> MTKYELKMQYFDEWMIRWRKFQTESDWEIEKGRQWWRRFNMAVSGALFCGLVLYTSGTATLKRQYGLPHF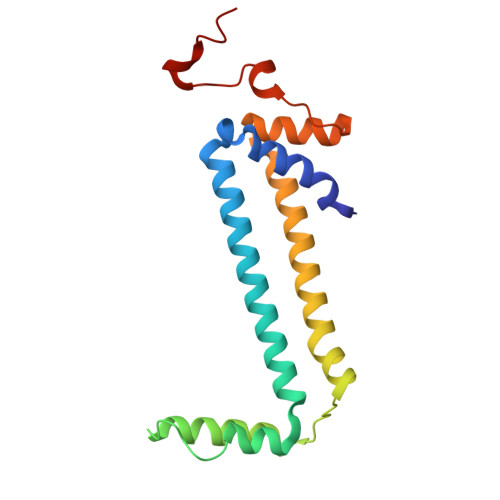FDIGVDGQAKETMLKTLTSRWRYTPQGYGRVLITGVPTYILFVTLEHYRERRRMQQYLQQNTVFGEQMRRLLSTGKIEEYLPVNIKATLPASQQAIYNY>[2x]MLDSKLKAPVFTVRTQGREYGEFVLEPLERGFGVTLGNPLRRILLSSIPGTAVTSVYIEDVLHEFSTIPGVKEDVVEIILNLKELVVRFLNPSLQTVTLLLKAEGPKEVKARDFLPVADVEIMNPDLHIATLEEGGRLNMEVRVDRGVGYVPAEKHGIKDRINAIPVDAVFSPVRRVAFQVEDTRLGQRTDLDKLTLRIWTDGSVTPLEALNQAVEILREHLTYFSNPQAAAVAAPEEAKEPEAPPEQEEELDLPLEELGLSTRVLHSLKEEGIESVRALLALNLKDLKNIPGIGERSLEEIKEALEKKGFTLKE;> MEIKRFGRIREVIPLPPLTEIQVESYRRALQADVPPEKRENVGIQAAFRETFPIEEEDKGKGGLVLDFLEYRLGEPPFPQDECREKDLTYQAPLYARLQLIHKDTGLIKEDEVFLGHIPLMTEDGSFIINGADRVIVSQIHRSPGVYFTPDPARPGRYIASIIPLPKRGPW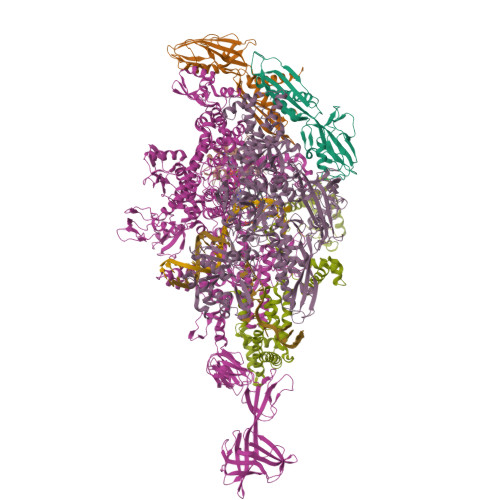IDLEVEPNGVVSMKVNKRKFPLVLLLRVLGYDQETLARELGAYGELVQGLMDESVFAMRPEEALIRLFTLLRPGDPPKRDKAVAYVYGLIADPRRYDLGEAGRYKAEEKLGIRLSGRTLARFEDGEFKDEVFLPTLRYLFALTAGVPGHEVDDIDHLGNRRIRTVGELMTDQFRVGLARLARGVRERMLMGSEDSLTPAKLVNSRPLEAAIREFFSRSQLSQFKDETNPLSSLRHKRRISALGPGGLTRERAGFDVRDVHRTHYGRICPVETPEGANIGLITSLAAYARVDELGFIRTPYRRVVGGVVTDEVVYMTATEEDRYTIAQANTPLEGNRIAAERVVARRKGEPVIVSPEEVEFMDVSPKQVFSVNTNLIPFLEHDDANRALMGSNMQTQAVPLIRAQAPVVMTGLEERVVRDSLAALYAEEDGEVAKVDGNRIVVRYEDGRLVEYPLRRFYRSNQGTALDQRPRVVVGQRVRKGDLLADGPASENGFLALGQNVLVAIMPFDGYNFEDAIVISEELLKRDFYTSIHIERYEIEARDTKLGPERITRDIPHLSEAALRDLDEEGVVRIGAEVKPGDILVGRTSFKGESEPTPEERLLRSIFGEKARDVKDTSLRVPPGEGGIVVRTVRLRRGDPGVELKPGVREVVRVYVAQKRKLQVGDKLANRHGNKGVVAKILPVEDMPHLPDGTPVDVILNPLGVPSRMNLGQILETHLGLAGYFLGQRYISPIFDGAKEPEIKELLAQAFEVYFGKRKGEGFGVDKREVEVLRRAEKLGLVTPGKTPEEQLKELFLQGKVVLYDGRTGEPIEGPIVVGQMFIMKLYHMVEDKMHARSTGPYSLITQQPLGGKAQFGGQRFGEMEVWALEAYGAAHTLQEMLTLKSDDIEGRNAAYEAIIKGEDVPEPSVPESFRVLVKELQALALDVQTLDEKDNPVDIFEGLASKR;> MKKEVRKVRIALASPEKIRSWSYGEVEKPETINYRTLKPERDGLFDERIFGPIKDYECACGKYKRQRFEGKVCERCGVEVTKSIVRRYRMGHIELATPAAHIWFVKDVPSKIGTLLDLSATELEQVLYFSKYIVLDPKGAILNGVPVEKRQLLTDEEYRELRYGKQETYPLPPGVDALVKDGEEVVKGQELAPGVVSRLDGVALYRFPRRVRVEYVKKERAGLRLPLAAWVEKEAYKPGEILAELPEPYLFRAEEEGVVELKELEEGAFLVLRREDEPVATYFLPVGMTPLVVHGEIVEKGQPLAEAKGLLRMPRQVRAAQVEAEEEGETVYLTLFLEWTEPKDYRVQPHMNVVVPEGARVEAGDKIVAAIDPEEEVIAEAEGVVHLHEPASILVVKARVYPFEDDVEVSTGDRVAPGDVLADGGKVKSDVYGRVEVDLVRNVVRVVESYDIDARMGAEAIQQLLKELDLEALEKELLEEMKHPSRARRAKARKRLEVVRAFLDSGNRPEWMILEAVPVLPPDLRPMVQVDGGRFATSDLNDLYRRLINRNNRLKKLLAQGAPEIIIRNEKRMLQEAVDALLDNGRRGAPVTNPGSDRPLRSLTDILSGKQGRFRQNLLGKRVDYSGRSVIVVGPQLKLHQCGLPKRMALELFKPFLLKKMEEKGIAPNVKAARRMLERQRDIKDEVWDALEEVIHGKVVLLNRAPTLHRLGIQAFQPVLVEGQSIQLHPLVCEAFNADFDGDQMAVHVPLSSFAQAEARIQMLSAHNLLSPASGEPLAKPSRDIILGLYYITQVRKEKKGAGLEFATPEEALAAHERGEVALNAPIKVAGRETSVGRLKYVFANPDEALLAVAHGIVDLQDVVTVRYMGKRLETSPGRILFARIVAEAVEDEKVAWELIQLDVPQEKNSLKDLVYQAFLRLGMEKTARLLDALKYYGFTFSTTSGITIGIDDAVIPEEKKQYLEEADRKLLQIEQAYEMGFLTDRERYDQILQLWTETTEKVTQAVFKNFEENYPFNPLYVMAQSGARGNPQQIRQLCGLRGLMQKPSGETFEVPVRSSFREGLTVLEYFISSHGARKGGADTALRTADSGYLTRKLVDVTHEIVVREADCGTTNYISVPLFQPDEVTRSLRLRKRADIEAGLYGRVLAREVEVLGVRLEEGRYLSMDDVHLLIKAAEAGEIQEVPVRSPLTCQTRYGVCQKCYGYDLSMARPVSIGEAVGIVAAQSIGEPGTQLTMRTFHTGGVAGAADITQGLPRVIELFEARRPKAKAVISEIDGVVRIEETEEKLSVFVESEGFSKEYKLPKEARLLVKDGDYVEAGQPLTRGAIDPHQLLEAKGPEAVERYLVEEIQKVYRAQGVKLHDKHIEIVVRQMMKYVEVTDPGDSRLLEGQVLEKWDVEALNERLIAEGKTPVAWKPLLMGVTKSALSTKSWLSAASFQNTTHVLTEAAIAGKKDELIGLKENVILGRLIPAGTGSDFVRFTQVVDQKTLKAIEEARKEA;> MAEPGIDKLFGMVDSKYRLTVVVAKRAQQLLRHGFKNTVLEPEERPKMQTLEGLFDDPNAVTWAMKELLTGRLVFGENLVPEDRLQKEMERLYPVEREE;> MKKSKRKNAQAQEAQETEVLVQEEAEELPEFPEGEPDPDLEDPDLTLEDDLLDLPEEGEGLDLEEEEEDLPIPKISTSDPVRQYLHEIGQVPLLTLEEEVELARKVEEGMEAIKKLSEITGLDPDLIREVVRAKILGSARVRHIPGLKETLDPKTVEEIDQKLKSLPKEHKRYLHIAREGEAARQHLIEANLRLVVSIAKKYTGRGLSFLDLIQEGNQGLIRAVEKFEYKRRFKFSTYATWWIRQAINRAIADQARTIRIPVHMVETINKLSRTARQLQQELGREPTYEEIAEAMGPGWDAKRVEETLKIAQEPVSLETPIGDEKDSFYGDFIPDEHLPSPVDAATQSLLSEELEKALSKLSEREAMVLKLRKGLIDGREHTLEEVGAFFGVTRERIRQIENKALRKLKYHESRTRKLRDFLD>GELVRTDSPNFLCSVLPTHWRCNKTLPIAFKVVAKGDVPDGTLVTVMAGNDENYSAELRNATAAMKNQVARF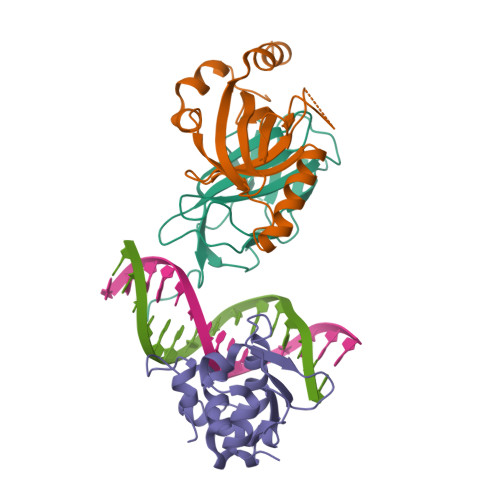NDLRFVGRSGRGKSFTLTITVFTNPPQVATYHRAIKITADGPREPRRHRQKLDDQTKPGSLSFSERLSELEQLRRTAMRVSPHHPAPTPNPRASLNHSTAFNPQPQSQMQDARQIQPSPPWSYDQSYQYLGS[2x];>[2x]MPRVVPDQRSKFENEEFFRKLSRECEIKYTGFRDRPHEERQTRFQNACRDGRSEIAFVATGTNLSLQFFPASWQGEQRQTPSREYVDLEREAGKVYLKAPMILNGVCVIWKGWIDLHRLDGMGCLEFDEERAQQEDALAQQA;>SLQRVPSYDSFDSEDYPAALPNHKPKGTFKDYVRDRADLNKDKPVIPAAALAGYTGSGPIQLWQFLLELLTDKSCQSFISWTGDGWEFKLSDPDEVARRWGKRKNKPKMNYEKLSRGLRYYYDKNIIHKTAGKRYVYRFVCDLQSLLGYTPEELHAMLDVKPDADE[2x]>MSLSLSHFRITRFQFARDRVIGDSQVRADDVNVAALELVSESGEVGLGFIQTLFNPLPDQQEIESVFEHEVWPSLKGNRAIALVHRVNRPRGGNQRAYSLPFHEAVQVALWDLAAKEAGLPLHVLLGSRRNRVKAYASGLDFHLDDDAFVSLFSHAASIGYSAFKIKVGHRDFDRDLRRLELLKTCVPAGSKVMIDPNEAWTSKEALTKLVAIREAGHDLLWVEDPILRHDHDGLRTLRHAVTWTQINSGEYLDLQGKRLLLEAHAADILNVHGQVTDVMRIGWLAAELGIP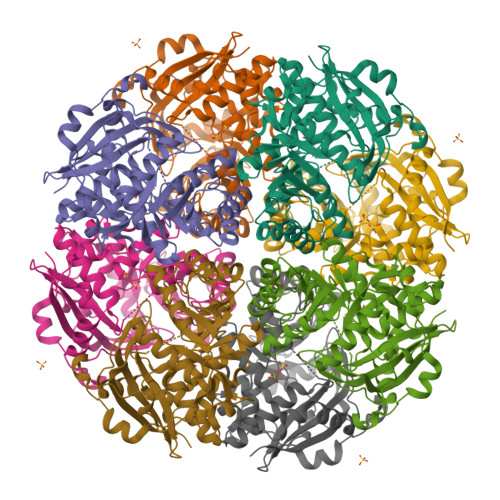ISIGNTFLEAGVHMAVALPEVEWLEYSFQNFDHLVEQPIEIRDGYAYAPDRPGHGLVLSEKARGEWSRPRRLARSELGAAPENPRLPAKEGHHHHHH[2x]(2E)-2-[(2S,4R)-5-[[[(2R,3S,4R,5R)-5-(6-aminopurin-9-yl)-3,4-bis(oxidanyl)oxolan-2-yl]methoxy-oxidanyl-phosphoryl]oxy-oxidanyl-phosphoryl]oxy-4-oxidanyl-3-oxidanylidene-pentan-2-yl]iminoethanoic acid | C17 H24 N6 O14 P2 | 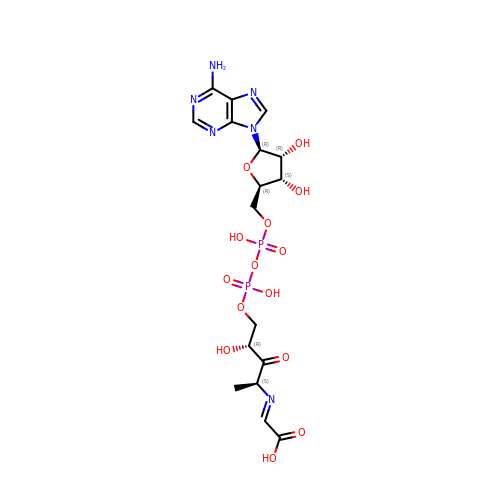DLIOKNCFMMUGKN-VGULMVRRSA-N> SNAMTNQDRPMKSMSESKCYKNRQVFPQ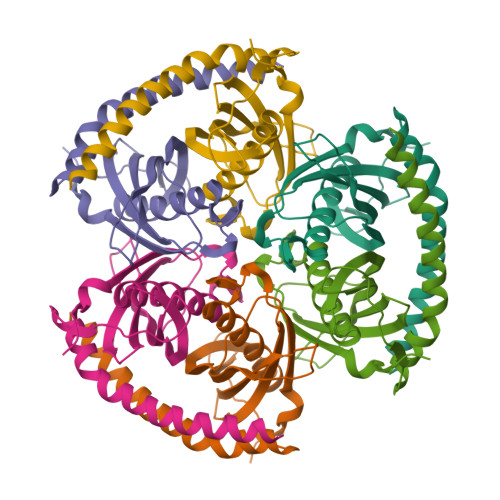DTAHHHTMFGGTLMANIDEIAAITAMKHAGAQVVTASTDSVDFLKPIKTGDILQYVAMVSYAGTSSMEVVVQIRIDDVFNNKHDLAALSYLTFVALDDEGKPKHVPGVYPEDDVEKWFYDTAPQRVERRKARRIESKQTIEYLAQAQHIRD> GDRVADMIESSIGNSVSRALTQALPAPTGQNTQVSSHRLDTGEVPALQAAEIGASSNTSDESMIETRCVLNSHSTAETTLDSFFSRAGLVGEIDLPLEGTTNPNGYANWDIDITGYAQMRRKVELFTYMRFDAEFTFVACTPTGQ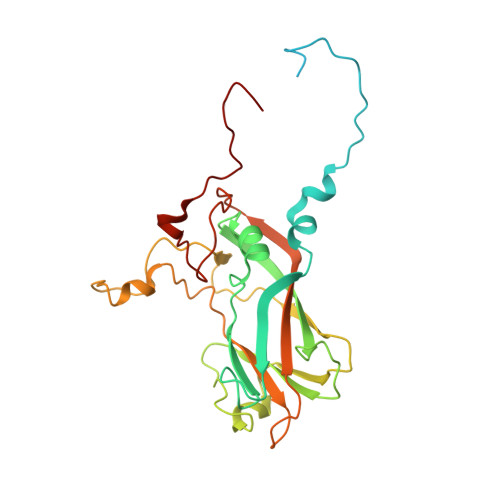VVPQLLQYMFVPPGAPKPESRESLAWQTATNPSVFVKLTDPPAQVSVPFMSPASAYQWFYDGYPTFGEHKQEKDLEYGACPNNMMGTFSVRTVGSSKSKYALVVRIYMRMKHVRAWIPRPMRNQNYLFKANPNYAGDSIKPTGTSRNAITTL> MIPGEYHVKPGQIALNTGRATCRVVVENHGDRPIQVGSHYHFAEVNPALKFDRQQAAGYRLNIPAG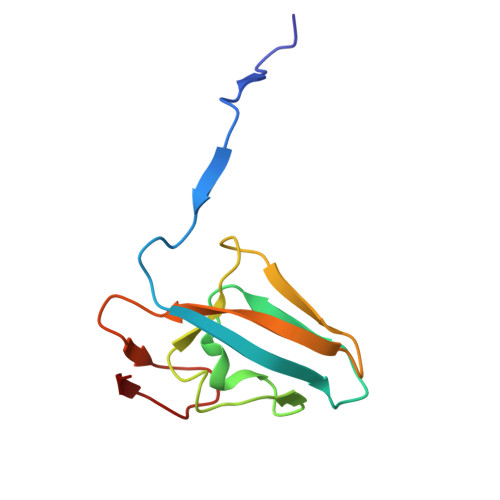TAVRFEPGQKREVELVAFAGHRAVFGFRGEVMGPL>[2x]GSMPFVNKQFNYRDPVNGVDIAYIKIPNAGQMQPVKAFKIHEGVWVIPERDTFTNPEEGDLNPPPEAKQVPVSYYDSTYLSTDNEKDNYLKGVIKLFDRIYSTGLGRMLLSFIVKGIPFWGGSTIDTELKVIDTNCINVIEPGGSYRSEELNLVITGPSADIIQFECKSFGHDVFNLTRNGYGSTQYIRFSPDFTFGFEESLEVDTNPLLGAGTFATDPAVTLAHQLIHAAHRLYGIAINPNRVLKVK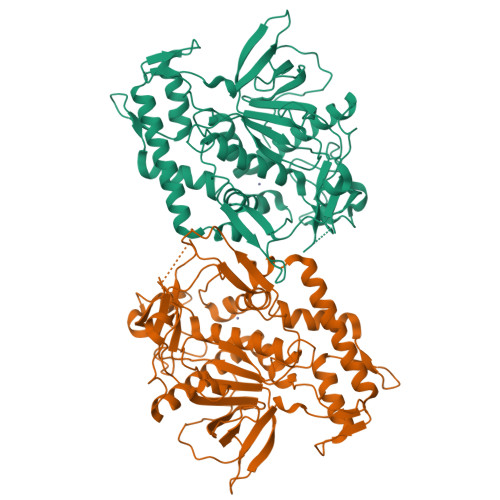TNAYYEMSGLEVSFEELRTFGGNDTNFIDSLWQKKFSRDAYDNLQNIARILNEAKTIVGTTTPLQYMKNIFIRKYFLSEDASGKISVNKAAFKEFYRVLTRGFTELEFVNPFKVINRKTFLNFDKAVFRINIVPDENYTINEGFNLEGANSNGQNTEINSRNFTRLKNFTG>[8x]MSIAESSVPIAVPVPTGGDDPTKVAMLGLTFDDVLLLPAASDVVPATADTSSQLTKRIRLRVPLVSSAMDTVTESRMAIAMARAGGMGVLHRNLPVAEQAGQVETVKRSEAGMVTDPVTCSPDNTLAEVDAMCARFRISGLPVVDDTGELVGIITNRDMRFEVDQSKPVSEVMTKA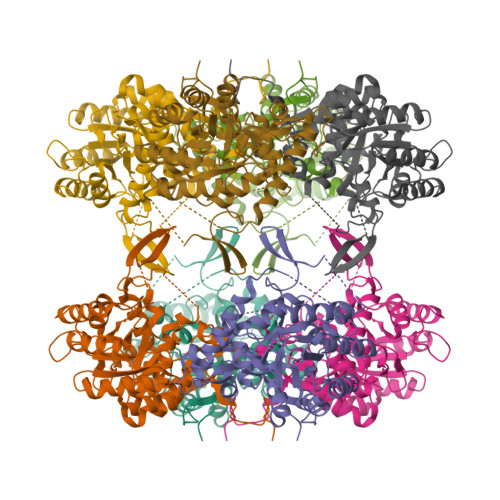PLITAKEGVSAEAALGLLRRHKIEKLPIVDGHGKLTGLITVKDFVKTEQFPLSTKDSDGRLLVGAAVGVGDDAWTRAMTLVDAGVDVLIVDTAHAHNRGVLDMVSRLKQAVGERVDVVGGNVATRAAAAALVEAGADAVKVGVGPGSICTTRVVAGVGAPQITAILEAVAACKPYGVPVIADGGLQYSGDIAKALAAGASTAMLGSLLAGTAESPGELIFVNGKQFKSYRGMGSLGAMQGRGAAKSYSKDRYFQDDVLSEDKLVPEGIEGRVPFRGPLGTVIHQLTGGLRAAMGYTGSATIEQLQQAQFVQITAAGLKESHPHDITMTVEAPNYYTR> GAMSGGLLKALRSDSYVELSQYRDQHFRGDNEEQEKL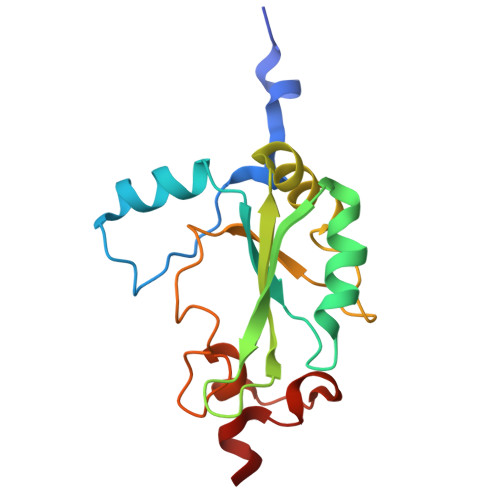LKKSCTLYVGNLSFYTTEEQIYELFSKSGDIKKIIMGLDKMKKTACGFCFVEYYSRADAENAMRYINGTRLDDRIIRTDWDAGFKEGRQYGRGRSGGQVRDEYRQDYDAGRGGYGKLAQNQ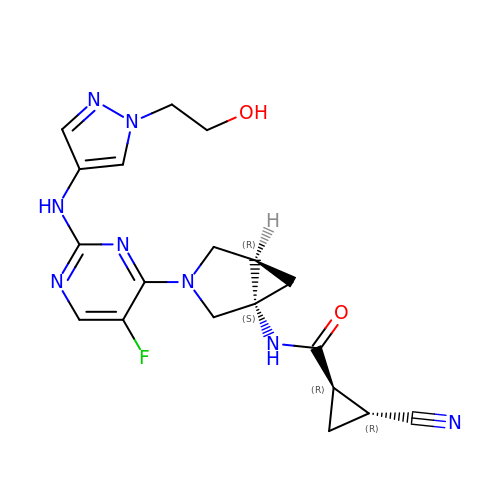(1R,2R)-2-cyano-N-[(1S,5R)-3-(5-fluoro-2-{[1-(2-hydroxyethyl)-1H-pyrazol-4-yl]amino}pyrimidin-4-yl)-3-azabicyclo[3.1.0]hexan-1-yl]cyclopropane-1-carboxamide | C19 H21 F N8 O2 | OCNRQCROIYCWQL-QULAYQROSA-N> MVEDELALFDKSINEFWNKFKSTDTSCQMAGLRDTYKDSIKAFAEKLSVKLKEEERMVEMFLEYQNQISRQNKLIQEKKDNLLKLIAEVKGKKQELEVLTANIQDLKEEYSRKKETISTANKANAERLKRLQKSADLYKDRLGLEIRKIYGEKLQFIFTNIDP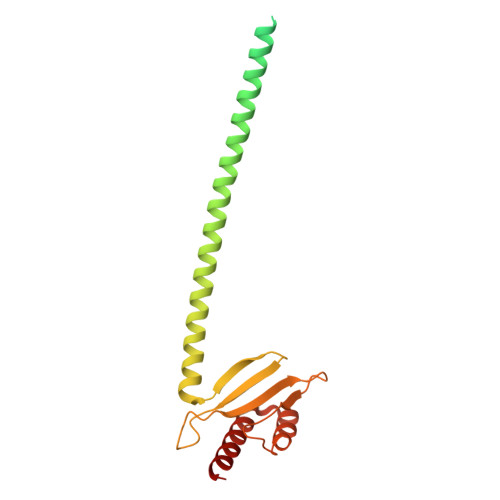KNPESPFMFSLHLNEARDYEVSDSAPHLEGLAEFQENVRKTNNFSAFLANVRKAFTATVYN> GGSTGGVPIQKVQDDTKTLIKTIVTRINDISHTQSVSAKQRVTGLDFIPGLHPILSLSKMDQTLAVYQQVLTSLPSQNVLQIANDLENLRDLLHLLAFSKSCSLPQTSGLQKPESLDGVLEASLYSTEVVALSRLQGSLQDILQQLDVSPEC;>AHHHHHHPGGPGSDELDLNLAYPISPWKFKLFCGPPNTTDDSFLSPAGAPNNASALKGASEAIVEAKFNSSGIYVPELSKTVFHCCFGNEQGQNCSALTDNTEGKTLASVVKASVFRQLGVNWDIECWMKGDLTLFICHMEPLPKNPFKNYDSKVHLLYDLPEVIDDSPLPPLKDSFQTVQCNCSLRGCECHVPVPRAKLNYALLMYLEITSAGVSFQSPLMSLQPMLVVKPDPPLGLHMEVTDDGNLKISWDSQTMAPFPLQYQVKYLENSTIVREAAEIVSATSLLVDSVLPGSSYEVQVRSKRLDGSGVWSDWSSPQVFTTQDVVYFPPKILTSVGSNASFHCIYKNENQIISSKQIVWWRNLAEKIPEIQYSIVSDRVSKVTFSNLKATRPRGKFTYDAVYCCNEQACHHRYAELYVIDVNINISCETDGYLTKMTCRWSPSTIQSLVGSTVQLRYHRRSLYCPDSPSIHPTSEPKNCVLQRDGFYECVFQPIFLLSGYTMWIRINHSLGSLDSPPTCVLPDSVVKPLPPSNVKAEITVNTGLLKVSWEKPVFPENNLQFQIRYGLSGKEIQWKTHEVFDAKSKSASLLVSDLCAVYVVQVRCRRLDGLGYWSNWSSPAYTLVMDVKVP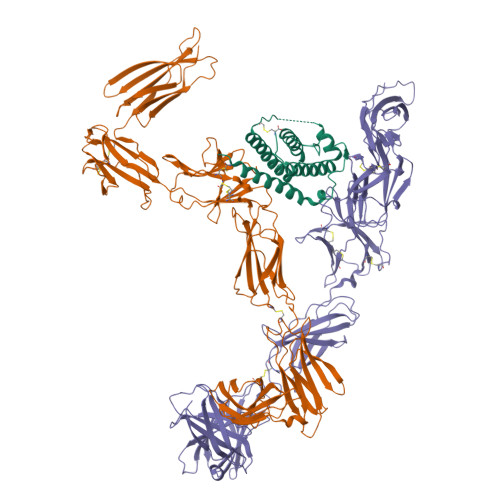MRGPEFWRKMDGDVTKKERNVTLLWKPLTKNDSLCSVRRYVVKHRTAHNGTWSEDVGNRTNLTFLWTEPAHTVTVLAVNSLGASLVNFNLTFSWPMSKVSAVESLSAYPLSSSCVILSWTLSPDDYSLLYLVIEWKILNEDDGMKWLRIPSNVKKFYIHDNFIPIEKYQFSLYPVFMEGVGKPKIINGFTKDAIDKQQNDAG[2x]>SNAMRNPNDVFHLAIPARDLDEAYDFYVTKLGCK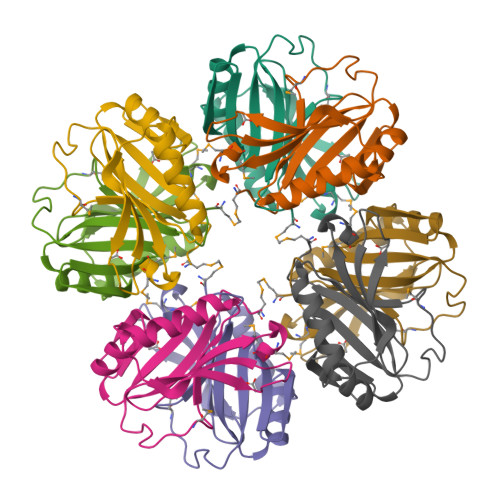LARRYPDRITLDFFGDQLVCHLSDRWDREVSMYPRHFGITFRDKKHFDNLYKLAKQRGIPFYHDLSRRFEGLIEEHETFFLIDPSNNLLEFKYYFDDRMMY[2x]> GSDEIDLSALRDPAGIFELVELVGNGTYGQVYKGRHVKTGQLAAIKVMDVTGDEEEEIKQEINMLKKYSHHRNIATYYGAFIKKNPPGMDDQLWLVMEFCGAGSVTDLIKNTKGNTLKEEWIAYICREILRGLSHLHQHKVIHRDIKGQNVLLTENAEVKLVDFGVSAQLDRTVGRRNTFIGTPYWMAPEVIACDENPDATYDFKSD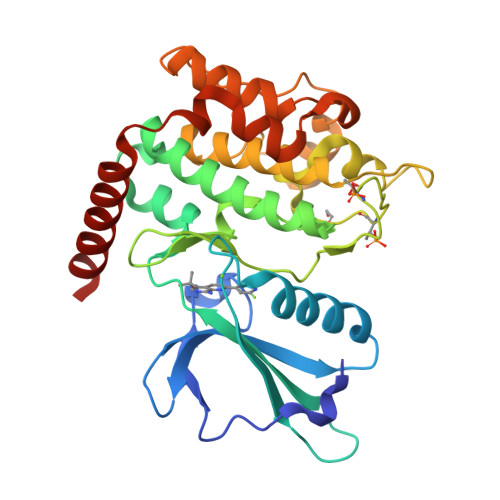LWSLGITAIEMAEGAPPLCDMHPMRALFLIPRNPAPRLKSKKWSKKFQSFIESCLVKNHSQRPATEQLMKHPFIRDQPNERQVRIQLKDHIDRTKKKRG(2E,5R)-5-(2-cyclohexylethyl)-5-{[(1S,3R)-3-(cyclopentylamino)cyclohexyl]methyl}-2-imino-3-methylimidazolidin-4-one | C24 H42 N4 O | 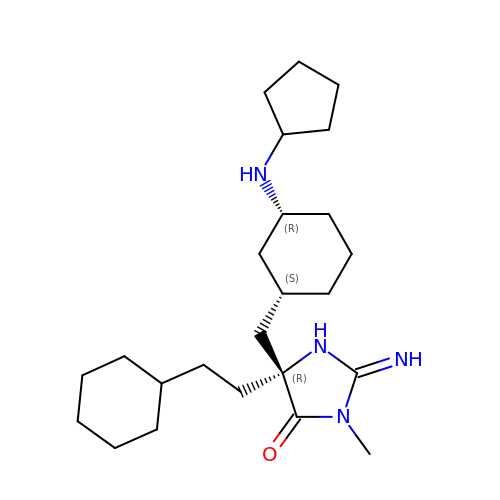NOZCXTAZEGFFAQ-XZDHIHRUSA-N> GGIAIYWGQNGNEGTLTQTCSTRKYSYVNIAFLNKFGNGQTPQINLAGHCNPAAGGCTIVSNGIRSCQIQGIKVMLSLGGGIGSYTLASQADAKNVADYLWNNF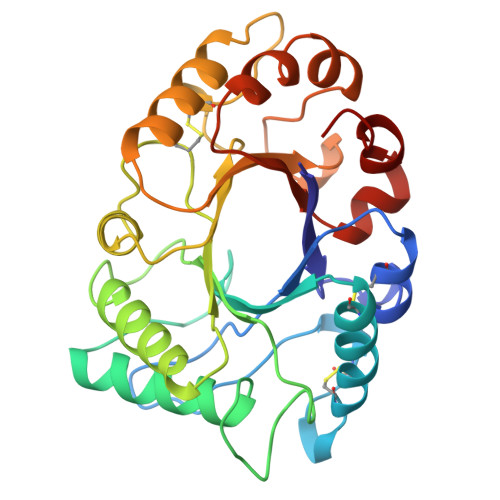LGGKSSSRPLGDAVLDGIDFDIEHGSTLYWDDLARYLSAYSKQGKKVYLTAAPQCPFPDRYLGTALNTGLFDYVWVQFYNNPPCQYSSGNINNIINSWNRWTTSINAGKIFLGLPAAPEAAGSGYVPPDVLISRILPEIKKSPKYGGVMLWSKFYDDKNGYSSSILDSV> MDYKDDDDKSVLITGVGVVAPNGLGLAPYWSAVLDGRHGLGPVTRFDVSRYPATLAGQIDDFHAPDHIPGRLLPQTDPSTRLALTAADWALQDAKADPESLTDYDMGVVTANACGGFDFTHREFRKLWSEGPKSVSVYESFAWFYAVNTGQISIRHGMRGPSSALVAEQAGGLDALGHARRTIRRGTPLVVSGGVDSALDPWGWVSQIASGRISTATDPDRAYLPFDERAAGYVPGEGGAILVLEDSAAAEARGRHDAYGELAGCASTFDPAPGSGRPAGLERAIRLALNDAGTGPEDVDVVFADGAGVPELDAAEARAIGRVFGREGV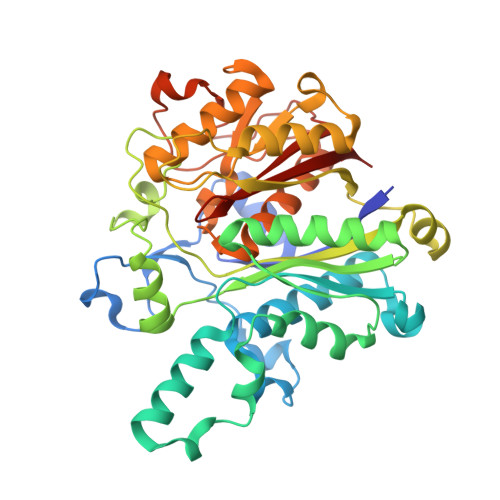PVTVPKTTTGRLYSGGGPLDVVTALMSLREGVIAPTAGVTSVPREYGIDLVLGEPRSTAPRTALVLARGRWGFNSAAVLRRFAPTP>MAANMYRVGDYVYFENSSSNPYLIRRIEELNKTANGNVEAKVVCFYRRRDISSTLIALADKHATLSVCYKAGPGADNGEEGEIEEEMENPEMVDLPEKLKHQLRHRELFLSRQLESLPATHIRGKCSVTLLNETESLKSYLEREDFFFYSLVYDPQQKTLLADKGEIRVGNRYQADITDLLKEGEEDGRDQSRLETQVWEAHNPLTDKQIDQFLVVARSVGTFARALDCSSSVRQPSLHMSAAAASRDITLFHAMDTLHKNIYDISKAISALVPQGGPVLCRDEMEEWSASEANLFEEALEKYGKDFTDIQQDFLPWKSLTSIIEYYYMWKTTDRYVQQKRLKAAEAESKLKQVYIPNYNKPNPNQISVNNVKAGVVNGTGAPGQSPGAGRACESCYTTQSYQWYSWGPPNMQCRLCASCWTYWKKYGGLKMPTRLDGERPGPNRSNMSPHGLPARSSGSPKFAMKTRQAFYLHTTKLTRIARRLCREILRPWHAARHPYLPINSAAIKAECTARLPEASQSPLVLKQAVRKPLEAVLRYLETHPRPPKPDPVKSVSSVLSSLTPAKVAPVINNGSPTILGKRSYEQHNGVDGNMKKRLLMPSRGLANHGQARHMGPSRNLLLNGKSYPTKVRLIRGGSLPPVKRRRMNWIDAPDDVFYMATEETRKIRKLLSSSETKRAARRPYKPIALRQSQALPPRPPPPAPVNDEPIVIED[2x];>MAQTQGTRRKVCYYYDGDVGNYYYGQGHPMKPHRIRMTHNLLLNYGLYRKMEIYRPHKANAEEMTKYHSDDYIKFLRSIRPDNMSEYSKQMQRFNVGEDCPVFDGLFEFCQLSTGGSVASAVKLNKQQTDIAVNWAGGLHHAKKSEASGFCYVNDIVLAILELLKYHQRVLYIDIDIHHGDGVEEAFYTTDRVMTVSFHKYGEYFPGTGDLRDIGAGKGKYYAVNYPLRDGIDDESYEAIFKPVMSKVMEMFQPSAVVLQCGSDSLSGDRLGCFNLTIKGHAKCVEFVKSFNLPMLMLGGGGYTIRNVARCWTYETAVALDTEIP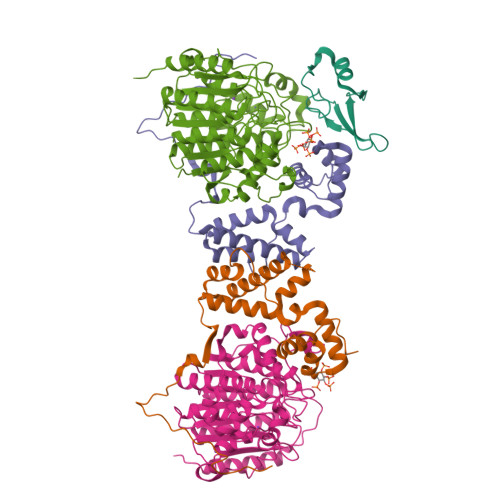NELPYNDYFEYFGPDFKLHISPSNMTNQNTNEYLEKIKQRLFENLRMLPHAPGVQMQAIPEDAIPEESGDEDEDDPDKRISICSSDKRIACEEEFSDSEEEGEGGRKNSSNFKKAKRVKTEDEKEKDPEEKKEVTEEEKTKEEKPEAKGVKEEVKLA[2x];> MRAHPGGGRCCPEQEEGESAAGGSGAGGDSAIEQGGQGSALAPSPVSGVRREGARGGGRGRGRWKQAGRGGGVCGRGRGRGRGRGRGRGRGRGRGRPPSGGSGLGGDGGGCGGGGSGGGGAPRREPVPFPSGSAGPGPRGPRATESGKRMDCPALPPGWKKEEVIRKSGLSAGKSDVYYFSPSGKKFRSKPQLARYLGNTVDLSSFDFRTGKMMPSKLQKNKQRLRNDPLNQNKGKPDLNTTLPIRQTASIFKQPVTKVTNHPSNKVKSDPQRMNEQPRQLFWEKRLQGLSASDVTEQIIKTMELPKGLQGVGPGSNDETLLSAVASALHTSSAPITGQVSAAVEKNPAVWLNTSQPLCKAFIVTDEDIRKQEERVQQVRKKLEEALMADILSRAADTEEMDIEMDSGDEA> MRSDKELKFLVVADFSTMRRIVRNLLKELGFNNVEEAEDGVDALNKLQAGGYGFVISDWNMPNMDGLELLKTIRADGAMSAL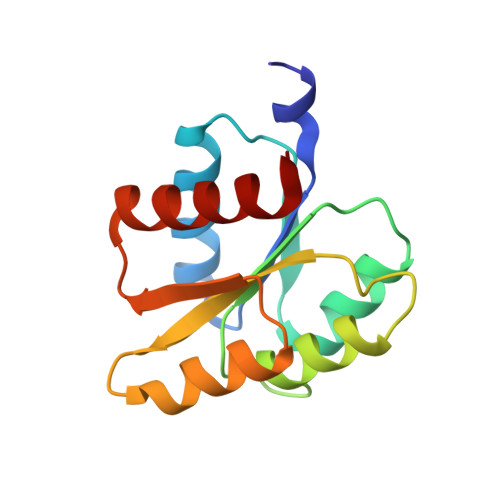PVLMVTAEAKKENIIAAAQAGASGYVVKPFTAATLEEKLNKIFEKLGM>MERIIQQTDYDALSCKLAAISVGYLPSSGLQRLSVDLSKKYTEWHRSYLITLKKFSRRAFGKVDKAMRSSFPVMNYGTYLRTVGIDAAILEFLVANEKVQVVNLGCGSDLRMLPLLQMFPHLAYVDIDYNESVELKNSILRESEILRISLGLSKEDTAKSPFLIDQGRYKLAACDLNDITETTRLLDVCTKREIPTIVISECLLCYMHNNESQLLINTIMSKFSHGLWISYDPIGGSQPNDRFGAIMQSNLKESRNLEMPTLMTYNSKEKYASRWSAAPNVIVNDMWEIFNAQIPESERKRLRSLQFL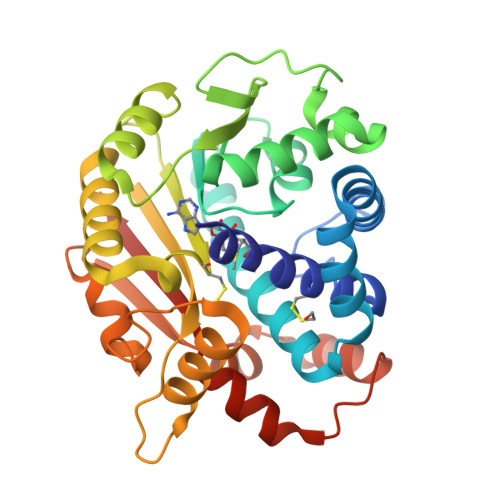DELEELKVMQTHYILMKAQWHHHHHH[3x]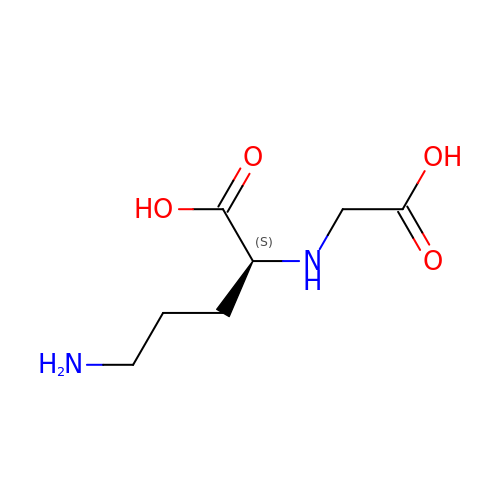(2~{S})-5-azanyl-2-(2-hydroxy-2-oxoethylamino)pentanoic acid | C7 H14 N2 O4 | YVSBHPGVGNJMHM-YFKPBYRVSA-N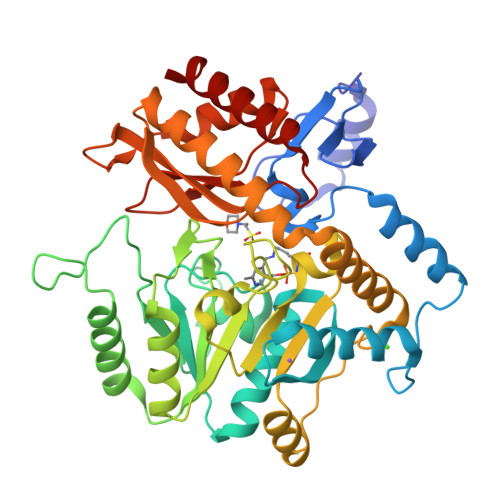> MSLNDDATFWRNARHHLVRYGGTFEPMIIERAKGSFVYDADGRAILDFTSGQMSAVLGHCHPEIVSVIGEYAGKLDHLFSEMLSRPVVDLATRLANITPPGLDRALLLSTGAESNEAAIRMAKLVTGKYEIVGFAQSWHGMTGAAASATYSAGRKGVGPAAVGSFAIPAPFTYRPRFERNGAYDYLAELDYAFDLIDRQSSGNLAAFIAEPILSSGGIIELPDGYMAALKRKCEARGMLLILDEAQTGVGRTGTMFACQRDGVTPDILTLSKTLGAGLPLAAIVTSAAIEERAHELGYLFYTTHVSDPLPAAVGLRVLDVVQRDGLVARANVMGDRLRRGLLDLMERFDCIGDVRGRGLLLGVEIVKDRRTKEPADGLGAKITRECMNLGLSMNIVQLPGMGGVFRIAPPLTVSEDEIDLGLSLLGQAIERAL> MDAENRVIINVGGIRHETYKATLKKIPATRLSRLTEGMLNYDPVLNEYFFDRHPGVFAQIINYYRSGKLHYPTDVCGPLFEEELEFWGLDSNQVEPCCWMTYT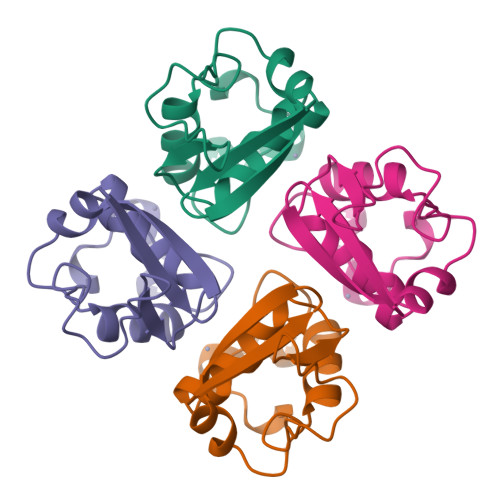AHRDTQETLAVL>[4x]SKIGINGFGRIGRLVLRTALEMGAQVVAVNDPFIALEYMVYMFKYDSTHGMFKGEVKVEDGALVVDGKKITVFNEMKPENIPWSKAGAEYIVESTGVFTTIEKASAHFKGGAKKVIISAPSADAPMFVCGVNLEKYSKDMKVVSNASCTTNCLAPVAKVLHENFEIVEGLMTTVHAVTATQKTVDGPSAKDWRGGRGAAQNIIPSSTGAAKAVGKVIPELDGKLTGM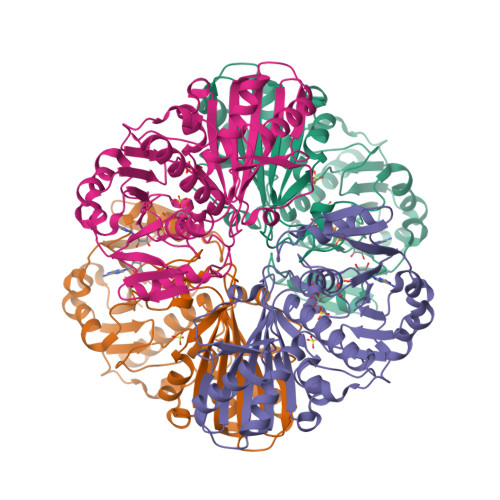AFRVPTPNVSVVDLTVRLGKECSYDDIKAAMKTASEGPLQGVLGYTEDDVVSCDFTGDNRSSIFDAKAGIQLSKTFVKVVSWYDNEFGYSQRVIDLIKHMQKVDSA> GMAKIEKNAPTMEKKPELFNIMEVDGVPTLILSKEWWEKVANFQAKPDDLILATYPKSGTTWMHEILDMILNDGDVEKCKRAQTLDRHAFLELKFPHKEKPDLEFVLEMSSPQLIKTHLPSHLIPPSIWKENCKIVYVARNPKDCLVSYYHFHRMASFMPDPQNLEEFYEKFMSGKVVGGSWFDHVKGWWAAKDMHRILYLFYEDIKKDPKREIEKILKFLEKDISEEILNKIIYHTSFDVMKQNPMTNYTTLPTSI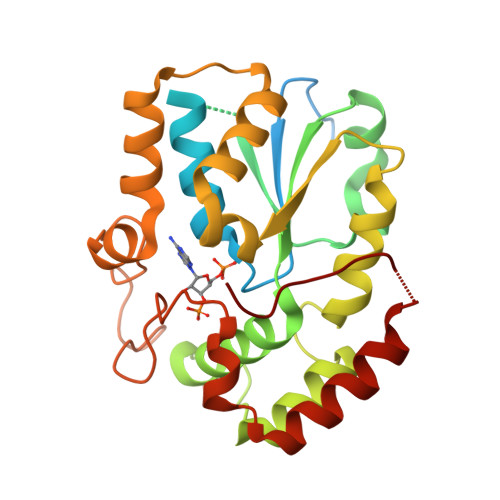MDHSISPFMRKGMPGDWKNYFTVAQNEEFDKDYQKKMAGSTLTFRTEI>[2x]LTAGLSVQQGIVRQRVIPVYQVNNLEEICQLIIQAFEAGVDFQESADSFLLMLCLHHAYQGDYKLFLESGAVKYLEGHGFRFEVKKRDGVKR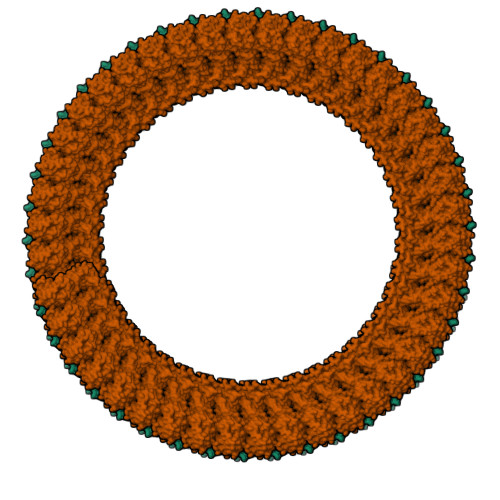LEELLPAVSSGKNIKRTLAAMPEEETTEANAGQFLSFASLFLPKLVVGEKACLEKVQRQIQVHAEQGLIQYPTAWQSVGHMMVIFRLMRTNFLIKFLLIHQGMHMVAGHDANDAVISNSVAQARFSGLLIVKTVLDHILQKTERGVRLHPLARTAKVKNEVNSFKAALSSLAKHGEYAPFARLLNLSGVNNLEHGLFPQLSAIALGVATAHGSTLAGVNVGEQYQQLREAATEAEKQLQQYAESRELDHLGLDDQEKKILMNFHQKKNEISFQQTNAMVTLRKERLAKLTEAITAASLPKTSGHYDDDDDIPFPGPINDDDNPGHQDDDPTDSQDTTIPDV> KC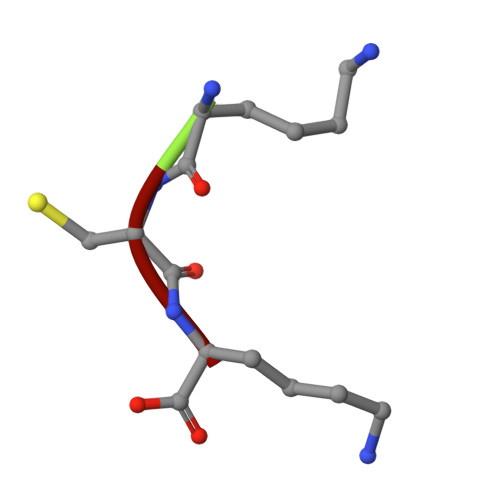K>[2x]SNAMIRKYRYGAPFDTEALTEKIETAEEAFPYGEISQKEGFAFTYIMDEDDIVYGLGESNRGINKRGYCYISNCTDDPIHTEDKRSLYGAHNFIIVSGKTTFGLFFDYPSKLTFDIGYTRMDTLKVSCENADLDIYVIEGENAYDIVKQFRRVIGRSYIPPKFAFGFGQSRYGYTTKEDFRA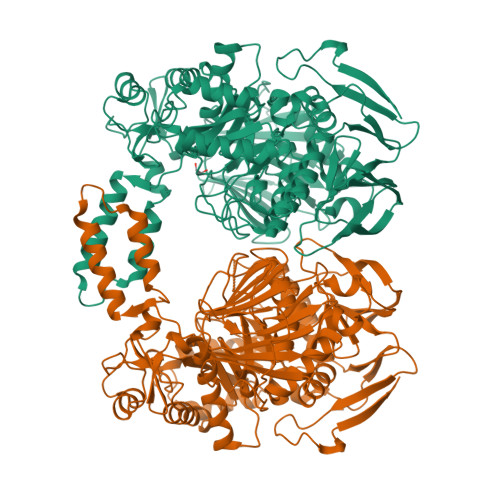VAKGYRENHIPIDMIYMDIDYMQDFKDFTVNEKNFPDFPEFVKEMKDQELRLIPIIDAGVKVEKGYEVYEEGVKNNYFCKREDGSDFVAAVWPGDTHFPDMLNPEARKWFGDKYRFLIDQGIEGFWNDMNEPAIFYSSEGLAEAKEFAGEFAKDTEGKIHPWAMQAKMKDIVNSPEDYKRFYHNVNGKKIRHDKVHNLFGYNMTRAAGEAFERIDPEKRFLMFSRSSYIGMHRYGGIWMGDNKSWWSHILLNLKMLPSLNMCGFMYTGADLGGFGDDTTRDLLLRFLALGVFTPLMRDHAAEGTREQECYQFENIEDFRSVINARYRLVPYLYSEYMKAALNDDMYFKPLGFVYPDDKMAIRVEDQLMLGNEIMIAPVYEQNARGRYVYLPEEMKFIKFMPDGSISEEVLEKGVHYVDVALNEVPLFIRSGKCIPVAEAAECVKDIDTENMQLIGYEGSSYTLYEDDGIHKDYDKKENYRVLTK> KTVHYLKDYQTPAYHILKTDLHFDINEPQTVVKSRLTVEPQRVGEPLVLDGSAKLLSVKINGAAADYVLEGETLTIAGVPSERFTVEVETEILPAENKSLMGLYASGGNLFTQCEPEGFRKITFYIDRPDVMSKFTTTIVADKKRYPVLLSNGNKIDGGEFSDGRHWVKWEDPFSKPSYLFALVAGDLAVTEDYFTTMSGRNVKIEFYTTEADKPKVGFAVESLKNAMKWDETRFGLEYDLDIFMVVAVGDFNMGAMENKGLNIFNTKFVLADSRTATDTDFEGIESVVGHEYFHNWTGNRVTCRDWFQLSLKEGLTVFRDQEFSGDRASRAVRRIENIRLLRQHQFPEDAGPTAHPVRPASYEEMNNFYTMTVYEKGAEVVRMYHTLLGEEGFQKGMKLYFQRHDGQAVTCDDFRAAMADANGINLDQFALWYSQAGTPVLEAEGRLKNNIFELTVKQTVPPTPDMTDKQPMM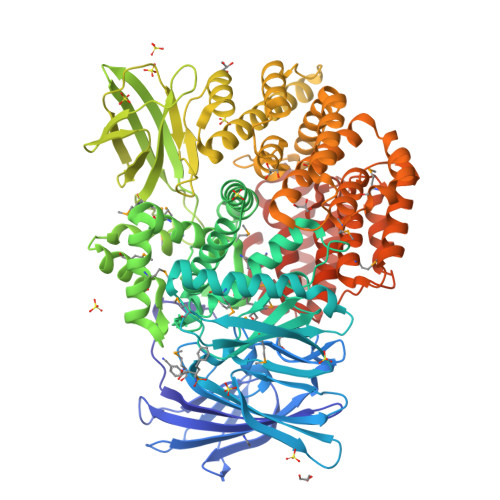IPVKVGLLNRNGEAVAFDYQGKRATEAVLLLTEAEQTFLLEGVTEAVVPSLLRGFSAPVHLNYPYSDDDLLLLLAHDSDAFTRWEAAQTLYRRAVAANLATLSDGVELPKHEKLLAAVEKVISDDLLDNAFKALLLGVPSEAELWDGAENIDPLRYHQAREALLDTLAVHFLPKWHELNRQAAKQENQSYEYSPEAAGWRTLRNVCRAFVLRADPAHIETVAEKYGEMAQNMTHEWGILSAVNGNESDTRNRLLAQFADKFSDDALVMDKYFALVGSSRRSDTLQQVRTALQHPKFSLENPNKARSLIGSFSRNVPHFHAEDGSGYRFIADKVIEIDRFNPQVAARLVQAFNLCNKLEPHRKNLVKQALQRIRAQEGLSKDVGEIVGKILDSNA> VMTMRGLLVGRMQPFHRGHLQVIKSILEEVDELIICIGSAQLSHSIRDPFTAGE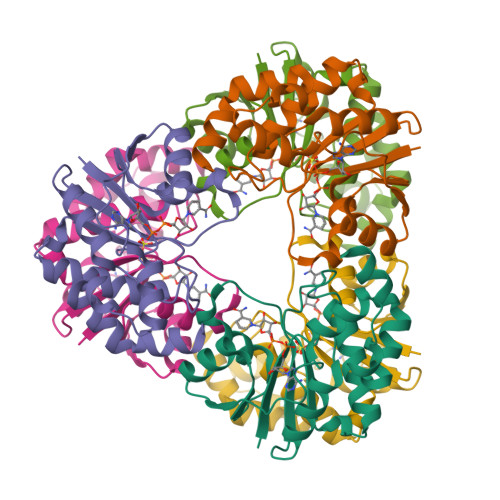RVMMLTKALSENGIPASRYYIIPVQDIECNALWVGHIKMLTPPFDRVYSGNPLVQRLFSEDGYEVTAPPLFYRDRYSGTEVARRMLDDGDWRSLLPESVVEVIDEINGVERIKHLAKKEVSELGGIS(4-chloranyl-1,3-thiazol-5-yl)methyl 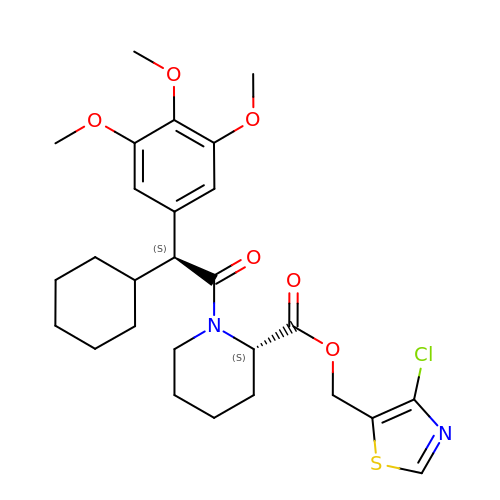(2S)-1-[(2S)-2-cyclohexyl-2-(3,4,5-trimethoxyphenyl)ethanoyl]piperidine-2-carboxylate | C27 H35 Cl N2 O6 S | BSUWGRNFALITMP-CVDCTZTESA-N>[2x]MQGVNIYNISAGTSVDLAAPVTTGDIVTFFSSALNLNAGAGNPNNTTLNLFAENGAYLLHIAFRLQENVIIFNSRQPDGPWLVEQRVSDVANQFAGIDGKAMVTVFDHGDKYQVVINEKTV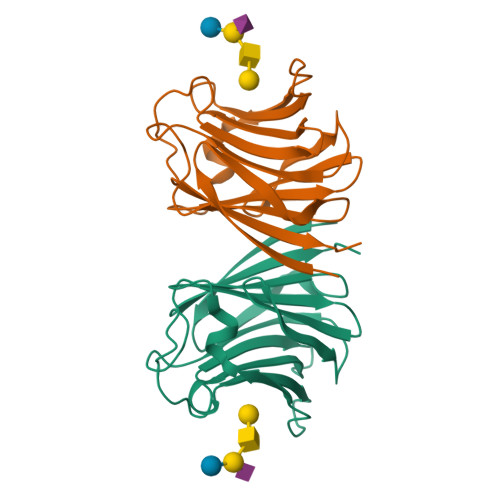IQYTKQISGLTSSLSYNATEETSIFSTVVEAVTYTGLA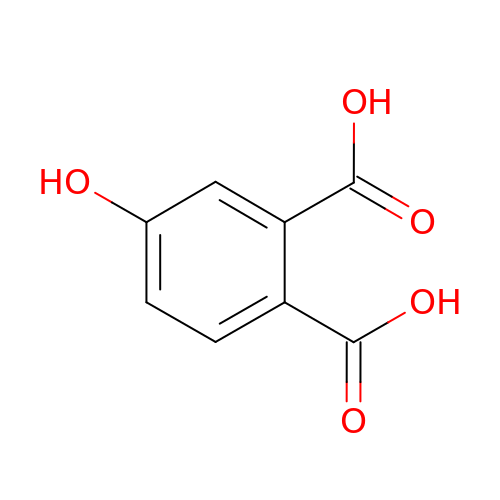4-hydroxybenzene-1,2-dicarboxylic acid | C8 H6 O5 | MWRVRCAFWBBXTL-UHFFFAOYSA-N>[2x]MGHHHHHHVIQWYPGHMAKAKREVSEQLKKVDVVFELVDARIPYSSRNPMIDEVINQKPRVVILNKKDMSNLNEMSKWEQFFIDKGYYPVSVDAKHGKNLKKVEAAAIKATAEKFEREKAKGL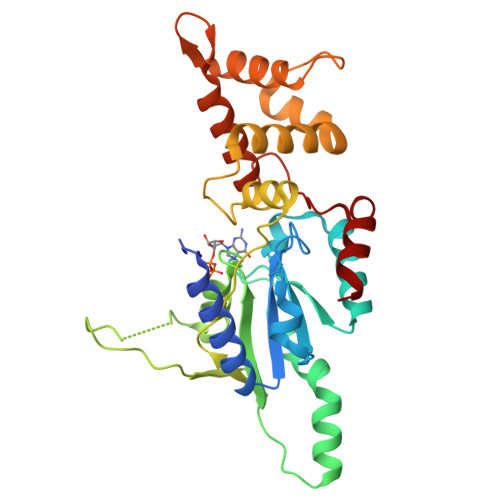KPRAIRAMIVGIPNVGKSTLINKLAKRSIAQTGNKPGVTKQQQWIKVGNALQLLDTPGILWPKFEDEEVGKKLSLTGAIKDSIVHLDEVAIYGLNFLIQNDLARLKSHYNIEVPEDAEIIAWFDAIGKKRGLIRRGNEIDYEAVIELIIYDIRNAKIGNYCFDIFKDMTEELANDANN NADPH oxidases (NOX) are transmembrane proteins, widely spread in eukaryotes and prokaryotes, that produce reactive oxygen species (ROS). The cytosolic dehydrogenase (DH) domain belongs to the Ferredoxin NADP +Reductase (FNR) family which has motifs to bind a flavin cofactor and a pyridine dinucleotide NAD(P)H. Thus, the NOX core catalytic domain contains the necessary machinery to move electrons from the electron donor – NADPH – through the flavin and heme cofactors to the ultimate electron acceptor, molecular oxygen, to make the ROS product. SpNOX purifies as a monomer and is constitutively active, so it represents the minimal functional core shared by all NOX family members. Here, we obtained X-ray structures of WT and F397W mutant of DH-only, and of a F397W mutant of full-length SpNOX.

We reasoned that changing the corresponding residue of SpNOX to W would stabilize FAD binding and inhibit NADPH binding, thereby reducing mobility of the two subdomains relative to each other. We interpreted this to mean that W in position 397 prevents hydride transfer by immobile stacking with the isoalloxazine ring of FAD, while W in position 399 has little effect on hydride transfer. De novo resolution at 1.94 Å of SpNOXDH F397W was possible because we co-crystallized in the presence of sodium bromide and collected a bromide-SAD dataset. As expected, SpNOXDH presents a typical fold of the FNR superfamily of reductase domain containing two sub-domains, the FAD-binding domain (FBD) and an NADPH-binding domain (NBD). In the asymmetric unit of SpNOXDH F397W, all molecules of the unit contain a well-defined FAD. These observations agree with flavin contents observed in solution and support the hypothesis that the F397W mutant stabilizes FAD binding. In contrast (and as predicted from the homologous FNR structure), the tryptophan of the F397W mutation makes an extensive and much tighter parallel stacking interaction at a distance of 3.5 Å from the isoalloxazine ring. Trp at position 397 appears to preclude access of the nicotinamide to the isoalloxazine, preventing direct hydride transfer. In line with conclusions from DH homologs, our data suggests that the SpNOX F397W sidechain represents the position that would be occupied by the nicotinamide ring of NADPH.

>[3x]QKISFPYLGKITHLKRLNHDTREIQIHLSRPFNYQSGQFAFLKIFQEGFESAPHPFSISGGHGQTLYFTVKTSGDHTKNIYDNLQAGSKVTLDRAYGHMIIEEGRENQVWIAGGIGITPFISYIREHPILDKQVHFYYSFRGDENAVYLDLLRNYAQKNPNFELHLIDSTKDGYLNFEQKEVPEHATVYMCGPISMMKALAKQIKKQNPKTELIYEGWKFK>MEEECRVLSIQSHVIRGYVGNRAATFPLQVLGFEIDAVNSVQFSNHTGYAHWKGQVLNSDELQELYEGLRLNNMNKYDYVLTGYTRDKSFLAMVVDIVQELKQQNPRLVYVCDPVLGDKWDGEGSMYVPEDLLPVYKEKVVPLADIITPNQFEAELLSGRKIHSQEEALRVMDMLHSMGPDTVVITSSDLPSPQGSNYLIVLGSQRRRNPAGSVVMERIRMDIRKVDAVFVGTGDLFAAMLLAWTHKHPNNLKVACEKTVSTLHHVLQRTIQCAKAQAGEGVRPSPMQLELRMVQSKRDIEDPEIVVQATVL[2x]

PL kinase is one of the key enzymes involved in PLP metabolism. In the presence of MgATP, this enzyme catalyzes the phosphorylation of the three inactive primary forms of vitamin B6, i.e. pyridoxine (PN), pyridoxamine (PM), and pyridoxal (PL) to their 5′-phosphorylated forms, PNP, PMP and PLP, respectively. PL kinase is a homodimer with each active site exclusively formed by a single monomer. The ATP binds in a shallow cavity at the active site, while the vitamin B6 substrate binds in a solvent-inaccessible deeper cavity opposite but facing the γ-phosphate of the ATP.

We also co-crystallized hPL kinase with ginkgotoxin (4′-O-methylpyridoxine) and MgATP, and the ternary complex structure was refined to 2.15 Å resolution. We observed bound MgATP and ginkgotoxin at both subunit active sites. The binding mode of MgATP is conserved as previously described for the wild-type hPL kinase-MgATP complex. The ATP β- and γ-phosphates are further stabilized by bound Mg2+ and Na+, the former ion being associated with both phosphate groups, while the Na+ is only associated with the γ-phosphate. The two molecules of ginkgotoxin are bound to the PL binding sites of the two enzyme monomers. We also observed what appears to be the phosphorylated product of ginkgotoxin bound at the PL sites, overlapping the bound unphosphorylated ginkgotoxin, although the electron density map showed a break in the ring structure and the phosphate moiety. Ginkgotoxin and its phosphorylated analog were refined with occupancies of 60% and 40%, respectively. The displacement of the ginkgotoxin phosphorylated analog toward ATP has placed its phosphate group about 3 Å from the ATP γ-phosphate group, as compared to the ∼6 Å closest distance between the ginkgotoxin C5′-OH and the ATP γ-phosphate. Like the hPL kinase D235A structure, we also observed a second bound Mg2+ at each active site that lies close to the ginkgotoxin phosphate and mediates an interaction with the ATP γ-phosphate, helping to dissipate the negative charges.>[2x]MLTLARQQQRQNIRWLLCLSVLMLLALLLSLCAGEQWISPGDWFTPRGELFVWQIRLPRTLAVLLVGAALAISGAVMQALFENPLAEPGLLGVSNGAGVGLIAAVLLGQGQLPNWALGLCAIAGALIITLILLRFARRHLSTSRLLLAGVALGIICSALMTWAIYFSTSVDLRQLMYWMMGGFGGVDWRQSWLMLALIPVLLWICCQSRPMNMLALGEISARQLGLPLWFWRNVLVAATGWMVGVSVALAGAIGFIGLVIPHILRLCGLTDHRVLLPGCALAGASALL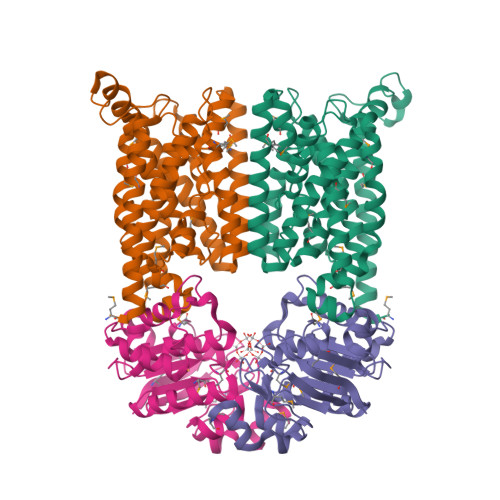LADIVARLALAAAELPIGVVTATLGAPVFIWLLLKAGR;>MSIVMQLQDVAESTRLGPLSGEVRAGEILHLVGPNGAGKSTLLARMAGMTSGKGSIQFAGQPLEAWSATKLALHRAYLSQQQTPPFATPVWHYLTLHQHDKTRTELLNDVAGALALDDKLGRSTNQLSGGEWQRVRLAAVVLQITPQANPAGQLLLLDEPMNSLDVAQQSALDKILSALCQQGLAIVMSSHDLNHTLRHAHRAWLLKGGKMLASGRREEVLTPPNLAQAYGMNFRRLDIEGHRMLISTI[2x]>SNAMKKFSVVIAGGGSTFTPGIVLMLLANQDRFPLRSLKFYDNDGARQETIAEACKVILKEQAPEIEFSYTTDPQAAFTDVDFVMAHIRVGKYPMREQDEKIPLRHGV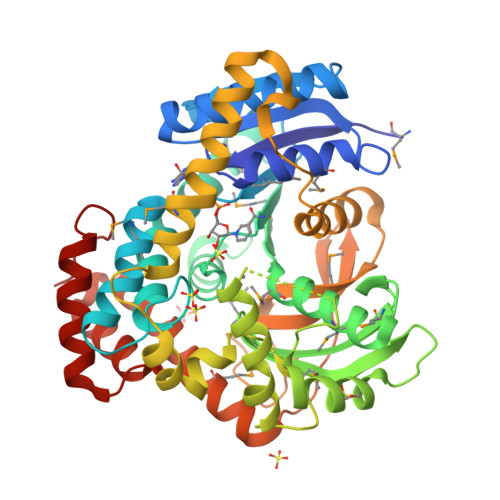LGQETCGPGGIAYGMRSIGGVLELVDYMEKYSPNAWMLNYSNPAAIVAEATRRLRPNAKILNICDMPIGIEGRMAQIVGLKDRKQMRVRYYGLNHFGWWTSIEDLDGNDLMPKLREYVAKYGYVPPSNDPHTEASWNDTFAKAKDVQALDPQTMPNTYLKYYLFPDYVVAHSNPERTRANEVMDHREKNVFSACRAIIAAGKSTAGDLEIDEHASYIVDLATAIAFNTQERMLLIVPNNGAIHNFDADAMVEIPCLVGHNGPEPLTVGDIPHFQKGLMSQQVAVEKLVVDAWEQRSYHKLWQAITLSKTVPSASVAKAILDDLIAANKDYWPELH[2x]> MDKINLVCGSLLHNIGKIIYRGTSERAKHSKLGGDFIKSFEQFRNTELTDCIRYHHAQEITSVKSNKEKNSLFYITYIADNISSGMDRRKDLEEGAEGFNWDKKVALGSVFNVLNEKEKGRQNYSYPFVARTRIKEEPLNFPTATQNQYTTSYYDGLITDMKTILQRLKPDKEHINSLLQMMESLWSYVPSSTDKNQLVDISLYDHSRTTAAIASAIYDYFQAENITDYQKELFDYNATEFYDKNAFLMMNFDMSGVQNFIYNISGSKALKSLRARSFYLDMLLEYISDNLLEKLELSRANILYVGGGHAYLLLANTNKTKAILSDFEHDLKTWFLDKFKIDLYVAMAYTEVSANDLMNHNGHYRDIYRRLSQKTSAKKANRYTAEEILNLNHQGTENARECRECKRSDLLIEEDDICEICDSLQKVSRDLTRENIFVIANEGVLDMPFGKKMSALSYSQADKLKKSNAEVQIYAKNISEIGQNLMTRIDMGDYTYRSDFHEMLEEVEVGINRLGVLRADVDNLGQAFINGIPDDYLSISRTATFSRAMSRFFKNYLNQLLAEKSYKINVIYAGGDDLFMIGAWQDILDFSIVLKQKFADFTQNKLSISAGIGMFREKYPVARMASLTGDLEDAAKDYKPDERAVQATKNAVTLFDATNVFSWDTLENDIFVKLDAITKNFEKLDETGKAFIYRLIDLLRGVNENQQINIARLAYTLSRMEEKIGKTFAQELYNWANADRKTLIMALEIYILKTRE;> MKIIKLYFESPVHFGEKRLSESKITFSADTLFSALMIEAVGLGKEDEFYQLASNNLVKFSDAFPFIDQYYYIPKPMFNLKLEKEDENPSKAFKKLLYVPIDSLEDYLSGGLDAYFERESFNLGKLALSEKVQQHDFKDSEPYNVGTFTFKENTGLYVLIEQTHPLLEELLENLQYSGIGGKRNSGYGKFKFEILEDSDIEDLFSAKGNRKILLSGALPKDAELEQALKNASYLLERRGGFVQSDTYATNLVKKQDLYVFKSGSTFENSFDGDIYQVGKKGNHPVYKYAKSFFLEVS;>[3x]TELKIGNEKVNSTNFGDFAEKAIRGINHKPFVNSKGGEQKITTSKIRGILELVNKVYNRVINTNDVELSENILADIAYIKVKIAYESGREPVVKDFIQRTAFTAAITDVMNQRTRESFLLFARYVESLIAYFKFYGGKD;>[4x]MKLVIEGTIVLKTGMHIGGSSDFSAIGAVASPVVRDTLTRLPLIPGSSLKGKMRYLLAKELNNGILLNEPNNDQDEILRLFGSSEKDKIRRARLKFNDIKLSNLAELETFNVSSTEVKFENTINRKTAVANPRQIERVIAGSKFDFEIFYNLDDIKEVEKDFENIKQGFDLLEFDYLGGHGTRGSGRIAFENLSVITAVGNFEKINTLNEILGA;> MKKTYRVTLTALGPIFIGGGEKLKKYEYIFDKQKKVAHMIDHTKFTKYLLEKNLLDDFTSRVNSHFDLYDYLVNKKGIVFMPLVKYSVPVAQFRTEVKNRFGKPISSPPMNDLNTFVKDAFGRPYIPGSSLKGALRTAILNDLKEDTKENEVFAHLQVSDSETIDLENLKVYQKVDYSKTAKPLPLYRECLKPNTEITFTVSFDDEYLTLKKIQNALHKTYQHYYIKWLKGGKVGETLIKGVYDSHADELKKNTFALDQPSQNQGEIIYIGGGAGFVSKTLHYKSKNRDQARNDSFDILKQLFRTTYSKMRSVPDNVPVALKLAVETKTFNGRVTGKHYLEMGKARIKLEEL

The multi-subunit Type III-A CRISPR-Cas effector complex (Csm) exemplifies this principle and is in addition regulated by cellular metabolites such as divalent metals and ATP. Recognition of the foreign or cognate target RNA (CTR) triggers its single-stranded deoxyribonuclease (DNase) and cyclic oligoadenylate (cOA) synthesis activities. The same activities remain dormant in the presence of the self or non-cognate target RNA (NTR) that differs from CTR only in its 3′-protospacer flanking sequence (3′-PFS). The single-stranded DNase (ssDNase) and the cOA synthesis activities reside within the Csm1 subunit and the RNase activity resides within Csm317–19.

Two distinct CTR-bound structures were resolved from two major classes that have 1123344151crRNA1Target1 (CTR-43) and 1122334151crRNA1Target1 (CTR-32) stoichiometry, respectively, where each number corresponds to a numbered Csm protein. Interestingly, unlike previously determined thermophilic Csm structures that prefer assemblies with fewer numbers of Csm3 and Csm224,25, LlCsm prefers the longer CTR-43. In contrast, though no ATP was used in formation of CTR-bound LlCsm, we observed 3′-PFS traversing through Csm1. Four nucleotides, C(-1)′-A(-2)′-A(-3)′-G(-4)′ of the 3′ PFS in CTR make a 90 degree turn from the trajectory of the rest of the target RNA and rests on Csm1. Notably, three helices: α12 of the Palm 1 domain, α17 and α21 of the Palm 2 domain of LlCsm1 point their N-terminal ends towards the phosphate backbone of the 3′ PFS nucleotides, thereby forming a positive groove that interacts favorably with the negatively charged 3′-PFS phosphate backbone in a sequence-independent manner. The 3′-PFS-helix dipole interaction locks the two Palm domains in preparation for Csm1-mediated activities. Four RNase centers are observed in the CTR-43 complex along the backbone of the bound CTR. The 2′-nucleophilic oxygen, the scissile phosphate group, and the leaving group oxygen form the classic inline geometry at each of the four sites. Either an arginine (sites 2–4) or a tyrosine (site 1) residue is situated near the 2′-nucleophilic oxygen that could act as the general base to extract the proton. A large number of particles of the CTR-43 but not those of the other two complexes lacked clearly defined side views of the HD domain, which could indicate a change in the structural property of the HD domain when CTR is bound.As an important member, 4-hydroxyphenylpyruvate dioxygenase (HPPD) catalyzes the complex transformation of 4-hydroxyphenylpyruvate acid (HPPA) to homogentisic acid (HGA), a key step in the tyrosine catabolic pathway that is common to all the aerobic organisms. In plants, HGA is a key intermediate in the biosynthesis of tocopherols and plastoquinones, which are essential compounds for the photosynthesis. Inhibition of the enzyme results in foliage bleaching of plants and eventually death, and thus HPPD inhibitors have been developed as herbicides for many years. Each monomeric unit consists of nine α-helices and sixteen β-strands that form two barrel-shaped structural domains: a conserved C-terminal domain containing the active site and a diversified N-terminal loop domain.

In this work, we successfully resolved the crystal structure of AtHPPD complexed with its natural substrate HPPA for the first time. The crystals belong to space group P 21 and comprise four molecules per asymmetric unit, which consists of two homodimers ( and ). Electron density for a ligand chelating with the metal ion was only seen in molecular A. The structure of HPPA can be built into the density map. Similarly, in HPPD-HPPA complex, the α-ketoglutarate moiety of HPPA in a bidentate interaction results in an octahedral coordination geometry involving the facial triad. In addition to chelation with metal ion, the phenolic hydroxyl of HPPA forms a hydrogen bond with the side chain of Asn423 on the C-terminal α-helix (α9). A 75° horizontal rotation, the benzene ring of HPPA shapes a T-π interaction with Phe381 and a weak hydrophobic interaction with the surrounding residues (such as Leu368 and Leu427, in ), leading to the current orientation of the aromatic moiety of HPPA. In the crystal structure, the values of D3 and D4 are 1.19 Å and 1.53 Å, which are more consistent with the structure of HPPD(Co2+)-HPPA(ketone), suggesting that the HPPA is more likely to be a ketone in the crystal. Besides, Gln293 underwent a conformation change during the binding of HPPA. More importantly, this conformation change made Gln293 involved in the formation of H-bond network of Ser267-Asn282-Gln307 which surrounds the HPPA in the active site. On the basis of the structural comparison, the remarkable characteristic of inactive state is the H-bond network formed by Glu394-Gln379-Asn423, whereas the key feature for the active state is the formation of the H-bond network by Ser267-Asn282-Gln307-Gln293.

>[4x]MGHQNAAVSENQNHDDGAASSPGFKLVGFSKFVRKNPKSDKFKVKRFHHIEFWCGDATNVARRFSWGLGMRFSAKSDLSTGNMVHASYLLTSGDLRFLFTAPYSPSLSAGEIKPTTTASIPSFDHGSCRSFFSSHGLGVRAVAIEVEDAESAFSISVANGAIPSSPPIVLNEAVTIAEVKLYGDVVLRYVSYKAEDTEKSEFLPGFERVEDASSFPLDYGIRRLDHAVGNVPELGPALTYVAGFTGFHQFAEFTADDVGTAESGLNSAVLASNDEMVLLPINEPVHGTKRKSQIQTYLEHNEGAGLQHLALMSEDIFRTLREMRKRSSIGGFDFMPSPPPTYYQNLKKRVGDVLSDDQIKECEELGILVDRDDQGTLLQIFTKPLGDRPTIFIEIIQRVGCMMKDEEGKAYQSGGCGGFGKGNFSELFKSIEEYEKTLEAKQLVG> MQEGAYRFIRNPNVSAEAIRKAGAMQTVKLAQEFPELLAIEDTTSLSYRHQVAEELGKLG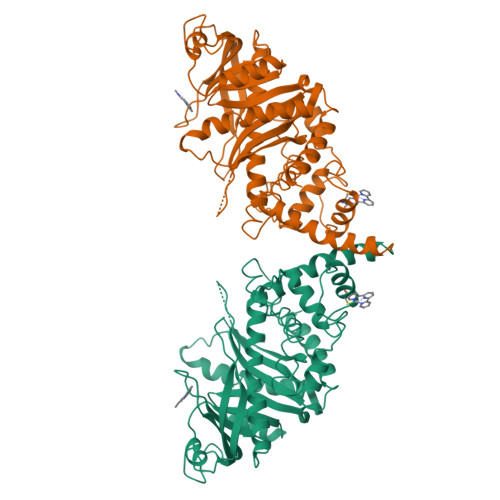SIQDKSRGWWVHSVLLLEATTFRTVGLLHQEWWMRPDDPADADEKESGKWLAAAATSRLRMGSMMSNVIAVCDREADIHAYLQDKLAHNERFVVRSKHPRKDVESGLYLYDHLKNQPELGGYQISIPQKGVVDKRGKRKNRPARKASLSLRSGRITLKQGNITLNAVLAEEINPPKGETPLKWLLLTSEPVESLAQALRVIDIYTHRWRIEEFHKAWKTGAGAERQRMEEPDNLERMVSILSFVAVRLLQLRESFTLPQALRAQGLLKEAEHVESQSAETVLTPDECQLLGYLDKGKRKRKEKGSLQWAYMAIARLGGFMDSKRTGIASWGALWEGWEALQSKLDGFLAAKDLMAQGIKI> QTLDIQRGATLFNRACAACHDTGGNIIQPGATLFTKDLERNGVDTEEEIYRVTYFGKGRMPGFGEKCTPRGQCTFGP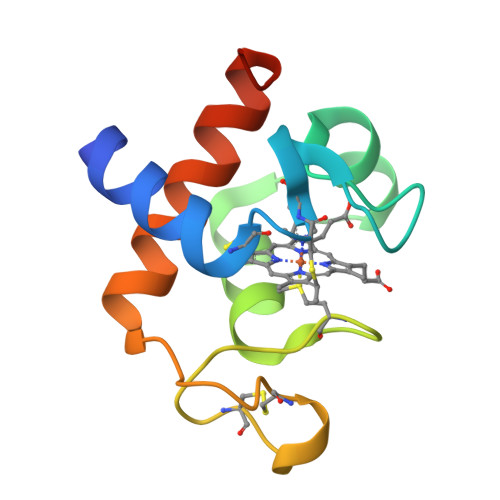RLQDEEIKLLAEFVKFQADQGWPTVSTD> KEKVKEPVKHLNSKNFDEFITKNKIVVVDFWAEWCAPCLILAPVIEELANDYPQVAFGKLNTEESQDIAMRYGIMSLPTIMFFKNGELVDQILGAVPREEIEV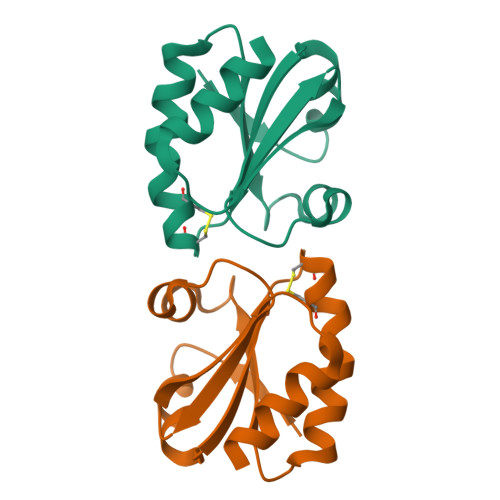RLKSLLE>SNADNSYKMDYPEMGLCIIINNKNFHKSTGMTSRSGTDVDAANLRETFRNLKYEVRNKNDLTREEIVELMRDVSKEDHSKRSSFVCVLLSHGEEGIIFGTNGPVDLKKITNFFRGDRCRSLTGKPKLFIIQACRGTELDCGIETASGVDDDMACHKIPVEADFLYAYSTAPGYYSWRNSKDGSWFIQSL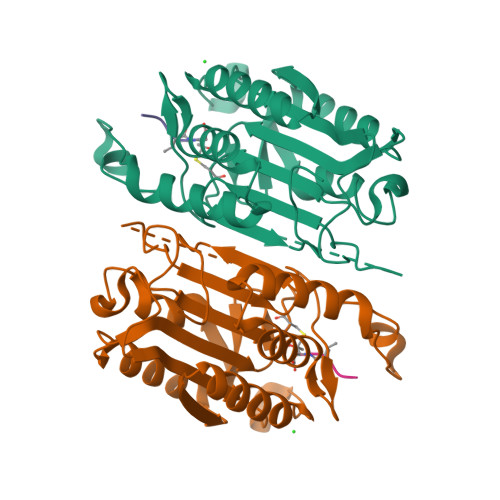CAMLKQYADKLEFMHILTRVNRKVATEFESFSFDATFHAKKQIPCIVSMLTKELYFYH[2x]>GIDPFTSTQQHTEPAEEETLHNIITDTENVQGSFSKHEFQAETKKLLDIVARSLYSEKEVFIRELISNGSDALEKLRHRMITAGGDTAPMEIHLQTDSVKGTFTIQDTGVGMNKEDLVSNLGTIARSGSKAFLDALQNQAEASSSIIGQFGVGFYSAFMVADKVEVYSQSAEADAPGYKWSSDGSGVFEVAEASGVRQGTKIVLHLKDDCKEFSSEDRVKEVVTKYSNFVSFPIFLNGRRLNTLQALWMMEPKDISEWQHEEFYRYVAQAYDKPRYTLHYRADAPLNIRSIFYVPEMKPSMFDVSREMGSSVALYSRKILIQTKATDILPKWLRFLRGVVDSEDIPLNLSRELLQESALIRKLRDVLQQRVIRFLLDQSKKDPEKYARFFEDYGLFMREGIVTTGEQSVKEDIAKLLRFESSALPAGQQTSLMEYSSRMKAGTRNIYYLCAPNRHLAEHSPYFEAMKQKDMEVLFCFEQFDELTLLHLREFDRKKLISAETDIVVDHYKEEKFQDSKPASERLSSEQAEDLLAWMRNALVQRVTNIKVTPRLDTHPAMITVLEMGAARHFLRTQQLARSSEERAQILQPTLEINTGHDLIKKLHALKDSNPELAQLLLEQIYDNAMIAAGLNEDPRPMISRLNQLLTRALEKH[2x]

Heat-shock protein 90 (Hsp90) is a highly conserved ATP-dependent molecular chaperone. Hsp90 is a V-shaped homodimer, with each protomer consisting of three major domains: a C-terminal dimerization domain (CTD); a middle domain (MD), which has been linked to client binding; and an N-terminal ATPase domain (NTD). Most higher eukaryotic cells possess four Hsp90 homologs: two cytosolic isoforms, one of which is constitutively expressed while the other is induced by heat shock and stress (Hsp90β and Hsp90α, respectively), one localized to the endoplasmic reticulum (Grp94) and one localized to the mitochondria (TRAP1). Using TRAP1 as a model system for Hsp90, here we investigate how ATP hydrolysis is coupled to its conformational asymmetry and propose a model connecting it to client remodeling.

To directly test the ability of the hemi-hydrolyzed dimer to exit the closed state, a FRET experiment was designed to look at the kinetics of dimer opening after ATP hydrolysis starting from a synchronized closed state population. This is possible because TRAP1 accumulates in the closed state upon addition of ATP in absence of Mg2+, whereupon hydrolysis can be initiated by addition of excess MgCl2. Wild-type zTRAP1 protein at 5 mg/mL in 50 mM HEPES pH 7.5, 50 mM KCl and 1 mM TCEP was incubated with 10 mM ATP and 10 mM EDTA for 1 hr at RT to allow TRAP1 closure before setting 2 µL hanging drops by mixing 1:1 with crystallization condition consisting of 0.2 M Na/K tartrate, 19% (v/v) PEG3350 and 36 mM hexammine cobalt. To differentiate between these possibilities, we took advantage of the fact that our crystals grow overnight, allowing collection and freezing of crystals every 24 hr for a time-resolved experiment. After screening crystals from multiple time points for diffraction quality, two additional datasets were collected (1-day and 53-day-old crystals), solved and refined through the same methods to resolutions of 3.5 Å and 2.2 Å, respectively. Similar to the 3-day-old crystal, no significant conformational differences were observed and no Mg2+ ion density was present in the ATP-binding pocket. However, electron densities for the ATP molecules showed a monotonic progression from an ATP-ATP structure (one day old crystal) through an ATP-ADP intermediate (3-day-old crystal) to an ADP-ADP structure (53-day-old crystal), clearly demonstrating that hydrolysis is occurring in the crystal. The fortuitous ability of the Mg2+-free closed state to be crystallized with ATP allowed the slow hydrolysis process to be examined crystallographically using crystals of different ages, revealing that the buckled protomer hydrolyzes ATP first while the straight protomer is still bound to an intact ATP. Ramachandran statistics for the refined zTRAP1 1-day structure are 94.6% favored, 5% allowed, 0.3% outlier.4-[(5,10-dimethyl-6-oxo-6,10-dihydro-5H-pyrimido[5,4-b]thieno[3,2-e][1,4]diazepin-2-yl)amino]benzenesulfonamide | C17 H16 N6 O3 S2 | 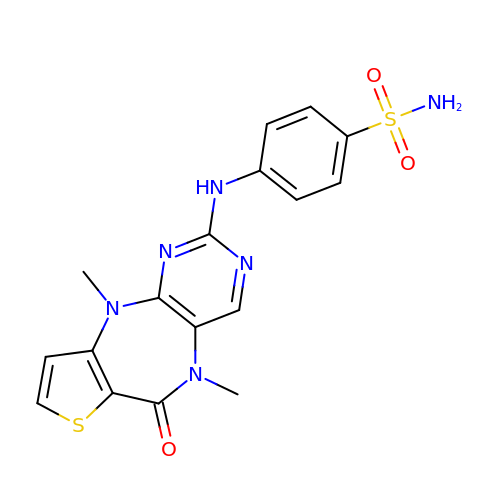YRDHKIFCGOZTGD-UHFFFAOYSA-N>[6x]SGMEVVLPLDPAVPAPLCPHGPTLLFVKVTQGAAATRRFYACSACRDRKDCNFFQWEDEKLSGARLAAREAHNRRCQPPLSRTQCVERYLKFIELPLTQRKFCQTCQQLLLPDDWGQHSEHQVLGNVSITQLRRPSQLLYPLENAATNAQYLFADRSCQFLVDLLSALGFRRVLCVGTPRLHELIKLTASGDKKSNIKSLLLDIDFRYSQFYME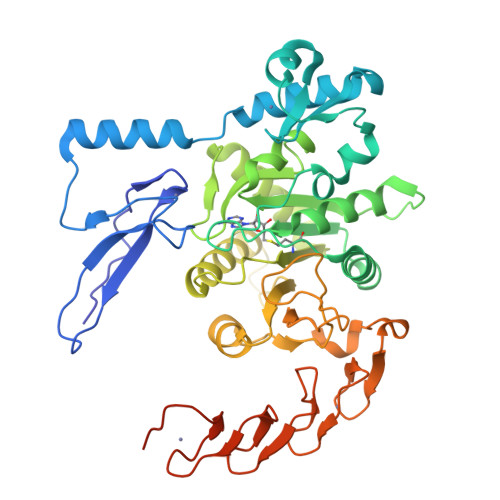DSFCHYNMFNHHFFDGKTALEVCRAFLQEDKGEGIIMVTDPPFGGLVEPLAITFKKLIAMWKEGQSQDDSHKELPIFWIFPYFFESRICQFFPSFQMLDYQVDYDNHALYKHGKTGRKQSPVRIFTNIPPNKIILPTEEGYRFCSPCQRYVSLENQHCELCNSCTSKDGRKWNHCFLCKKCVKPSWIHCSICNHCAVPDHSCEGPKHGCFICGELDHKRSTCPNIATS The bifunctional alcohol–acetaldehyde dehydrogenase enzyme (AdhE) is a key metabolic enzyme of the alcoholic fermentation pathway. AdhE converts acetyl-coenzyme A to acetaldehyde and then to ethanol, in a two-step reaction that is coupled with the oxidation of two NADH molecules into NAD+. Intriguingly, AdhE is capable of oligomerization and forms a filament (identified as spirosome in early studies).

Incubation with NAD+ and Fe2+ is sufficient to extend the filaments. Clear density for NAD+ and Fe2+ could be observed in the density map in the AlDH and ADH domains in both subunits of the AdhE dimer. The AdhE helical assembly can be described as one AdhE dimer repeated along a right-handed helix with a helical twist of 164.5 Å and a rise of 56.4 Å. In the extended AdhE filament, three different inter-domain interfaces are formed. The dimer is maintained through an AlDH–AlDH interface (named (α-AlDH)n/(β-AlDH)n interface) and two symmetric AlDH–ADH interfaces (named (α-AlDH)n/(β-ADH)n and (α-ADH)n/(β-AlDH)n interfaces). By superimposing these structures with AdhE, we could observe that the interfaces present in dimers of monofunctional enzymes correspond to the ADH–ADH and AlDH–AlDH interfaces of the extended spirosomes. Remarkably, the substrate/product channels of both the AlDH and ADH domains lead to the two cavities located at the AlDH–ADH interfaces within the AdhE dimer. The loops 2 and 3 seal this cavity by mediating the interactions between the AlDH and ADH domains. This allows a direct channeling between the AlDH and ADH domain active sites. Therefore, only extended filaments are bound to cofactors and are able to catalyze the two-step reaction of conversion of acetyl-CoA to ethanol.

>[4x]MAVTNVAELNALVERVKKAQREYASFTQEQVDKIFRAAALAAADARIPLAKMAVAESGMGIVEDKVIKNHFASEYIYNAYKDEKTCGVLSEDDTFGTITIAEPIGIICGIVPTTNPTSTAIFKSLISLKTRNAIIFSPHPRAKDATNKAADIVLQAAIAAGAPKDLIGWIDQPSVELSNALMHHPDINLILATGGPGMVKAAYSSGKPAIGVGAGNTPVVIDETADIKRAVASVLMSKTFDNGVICASEQSVVVVDSVYDAVRERFATHGGYLLQGKELKAVQDVILKNGALNAAIVGQPAYKIAELAGFSVPENTKILIGEVTVVDESEPFAHEKLSPTLAMYRAKDFEDAVEKAEKLVAMGGIGHTSCLYTDQDNQPARVSYFGQKMKTARILINTPASQGGIGDLYNFKLAPSLTLGCGSWGGNSISENVGPKHLINKKTVAKRAENMLWHKLPKSIYFRRGSLPIALDEVITDGHKRALIVTDRFLFNNGYADQITSVLKAAGVETEVFFEVEADPTLSIVRKGAELANSFKPDVIIALGGGSPMDAAKIMWVMYEHPETHFEELALRFMDIRKRIYKFPKMGVKAKMIAVTTTSGTGSEVTPFAVVTDDATGQKYPLADYALTPDMAIVDANLVMDMPKSLCAFGGLDAVTHAMEAYVSVLASEFSDGQALQALKLLKEYLPASYHEGSKNPVARERVHSAATIAGIAFANAFLGVCHSMAHKLGSQFHIPHGLANALLICNVIRYNANDNPTKQTAFSQYDRPQARRRYAEIADHLGLSAPGDRTAAKIEKLLAWLETLKAELGIPKSIREAGVQEADFLANVDKLSEDAFDDQCTGANPRYPLISELKQILLDTYYGRDYVEGETAAKKEAAPAKAEKKAKKSA> SRSFPLGIKQTLPRHILRATGDQPSSSSSMSALAAKPPKSPCSLSVDTCKDSSPSELVVYERRDGKRWVHRHQLSLYLSHAVGLGYFRAQFEDSSVTPAAVFDCLSHLVRPPVHAARSEEDEGDEGGERRQNKQVDGAPDGDGERVTAQDLSEFMKNCVASRYRDVDVLDVVTDVLSALLIGSADLPLLVDIASSCIALSLLRPKLFTAIASRLLVLLPPAPASGSSPLDAAALSPRQAVRLVESFSHQRFRHPDVLPLLFLSLSPSLPFLSPRLACRLLHAVAGLGACAAPAETVQLLLSRVASGLGDCVGRPGCESETHCQTATGDHRMIQQTSDLPESEFLEKQIQGQKLQPQLALAD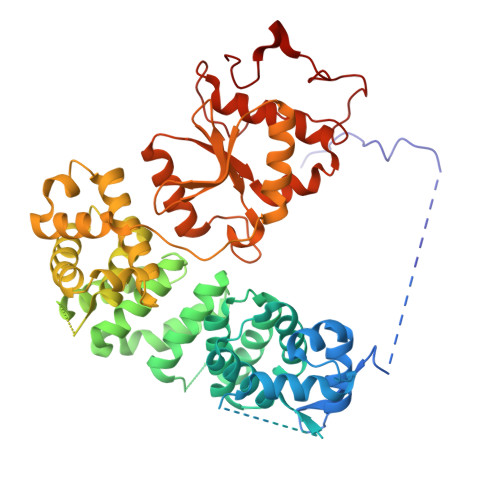LTKATHALLLLEIELEQKPLLESLLTAMAPEIFDHPVEFWSSSPAGPSLHRRLLLIRTALRHLHRDTIYNSLPTMVRQAFRRLHRIEITSPPRSPTHFVTRMSALLTRLRIAHFCYAIRGPLVFDVLERDRPIVWQCNTADRFYVNSAEKTTAVKLQERITQAMGLKVGNCEYWQWMKMKRKRTRLEYIRMQRYYILKDRRQHDPDFEGWTLPLVHHMHRRNRLHYDYYFPNYTPLSRVEY> MVPISPIETVPVKLKPGMDGPKVKQWPLTEEKIKALVEICTELEKEGKISKIGPENP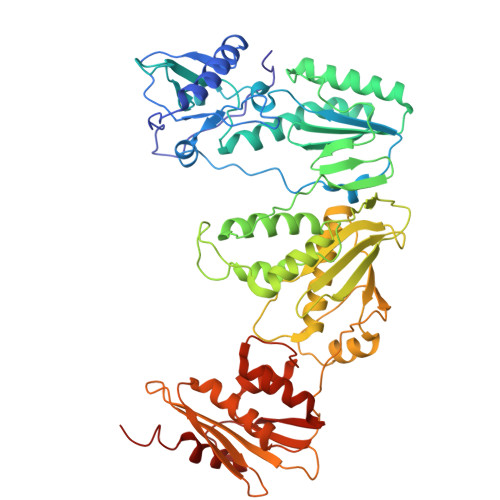YNTPVFAIKKKNSTRWRKLVDFRELNKRTQDFWEVQLGIPHPAGLKKKKSVTVLDVGDAYFSVPLDEDFRKYTAFTIPSINNETPGIRYQYNVLPQGWKGSPAIFQSSMTKILEPFKKQNPDIVIYQYMDDLYVGSDLEIGQHRTKIEELRQHLLRWGLYTPDQKHQKEPPFLWMGYELHPDKWTVQPIVLPEKDSWTVNDICKLVGKLNWASQIYPGIKVRQLSKLLRGTKALTEVIPLTEEAELELAENREILKEPVHGVYYDPSKDLIAEIQKQGQGQWTYQIYQEPFKNLKTGKYARMRGAHTNDVKQLTEAVQKITTESIVIWGKTPKFKLPIQKETWETWWTEYWQATWIPEWEFVNTPPLVKLWYQLEKEPIVGAETFYVDGAANRETKLGKAGYVTNKGRQKVVPLTNTTNQKTELQAIYLALQDSGLEVNIVTDSQYALGIIQAQPDKSESELVNQIIEQLIKKEKVYLAWVPAHKGIGGNEQVDKLVSAGIRKVL>[2x]GMQTNSKIYIAGHKGTAGTALVENLQKRGFNNLVLKTRQELDLVNQQAVAKFFKEEKPEYVFLTAVLPCGAANVAQRADFIYENLMIQNNVIHNSFLNNVKKLVFFGSGYMYPENAKNPLKEEYLFQGDLEYGAYSFGAAKIAGAIMCESYNIQYGTNFITLVLNNLYGTKANFDFGKSRVLPALLRKFHLAKLLSEGNITQILQDLKMNNFEEAKEYLHNFGISKKSVEIWGTGKVRREFI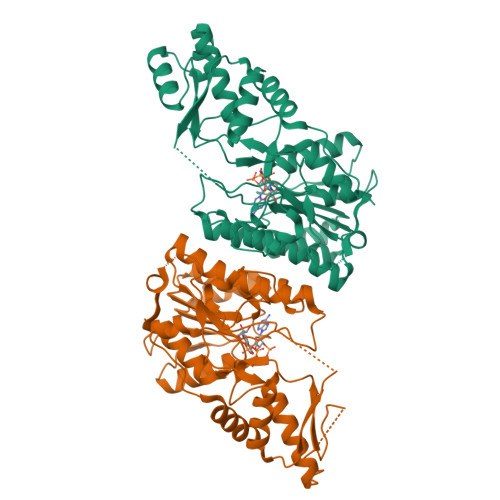HSDDLADVAIYTMQNIDFKDLIKDRKSKNTHINIGTGIDYSIKEVALMVKNIVGFSGELVFNTSRPDSTMDRLMDCSKIHSLGWKHKIELKDGIKMMYEWYKT(2R)-3-({[4-[(PYRIDIN-4-YL)PHENYL]-THIEN-2-YL}CARBOXAMIDO)(PHENYL)PROPANOIC 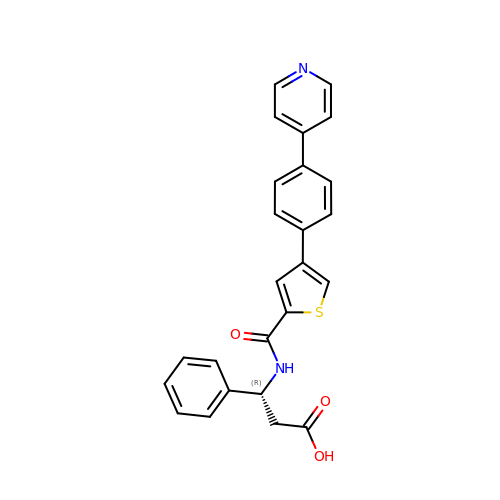ACID | C25 H20 N2 O3 S | VMTJQZUZINLEKC-JOCHJYFZSA-N Hook microtubule tethering protein 3 (Hook3), a cargo adaptor protein that serves as a crucial scaffold protein linking cargo to microtubule motors, plays a pivotal role in regulating bidirectional early endosome trafficking, managing directional movement, and maintaining Golgi morphology. Among these domains, the Hook domain together with the first and second coiled coils serve as the dynein-binding region, whereas the third coiled coil-containing the carboxyl-terminal region interacts with several proteins, including fused toes homolog (FTS), FTS−Hook−FHIP1B (FHF) complex subunit Hook interacting protein 1B (FHIP1B), and kinesin family member 1 C (KIF1C). KIF1C, a kinesin-3 family member with plus-end-directed motility, mediates the anterograde (plus-end-directed) transport of vesicles containing several components, such as α5β1 integrin, 14-3-3, and protein tyrosine phosphatase non-receptor type 21 (PTPN21). A previous study showed that KIF1C exists as an autoinhibited homodimer, and becomes activated by interacting with the carboxyl-terminal region of Hook3 or the FERM domain of PTPN21.

Next, we attempted to crystallize Hook3(553–624) and KIF1C(714–809), separately and as a complex (marked in red). The crystal structures of Hook3(553–624) in an apo form (Fig. EV1A) and in a complex with KIF1C(714–809) were determined to resolutions of 2.7 Å and 3.0 Å, respectively (Table EV1). Even though Hook3 exists in a parallel coiled-coil form in both structures (Figs. 2B and EV1A), the two Hook3 structures did not exactly match up when superimposed (Fig. EV1B).

>GHMEKLHEANNELQKKRAIIEDLEPRFNNSSLKIEELQEALRKKEEEMKQMEERYKKYLEKAKSVIRTLDPKQNQ[2x]> GAMVSPSLIA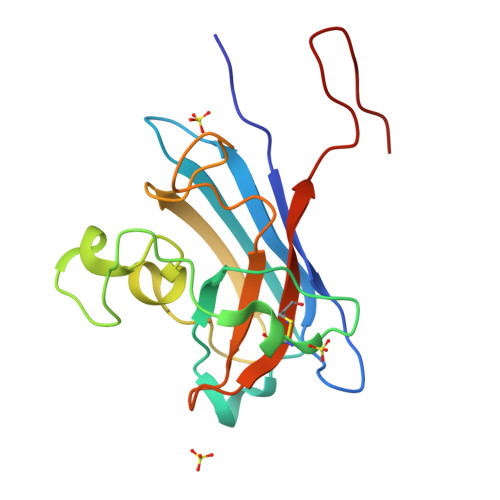KFEKTSKSNIEGTIKFTPANNGTVSVSVDLKGLPSDIGPFPYHVHEKPVPASKNCSATENHFNPYNGTVRAATPAAHAVGDLAGKHGNIMGESYKTEYDDSYISLNEKSRSYIGGLSIVIHANNGTRLNCANITLLDEGHGNANTTMSN5-{2-[2-(2,4-dioxo-3,4-dihydropyrimidin-1(2H)-yl)ethoxy]-4-fluorophenoxy}-7-fluoronaphthalene-2-carbonitrile | C23 H15 F2 N3 O4 | 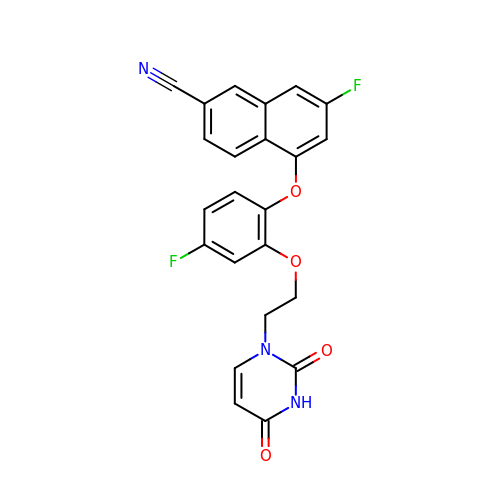RQCNWTHUESPRKJ-UHFFFAOYSA-N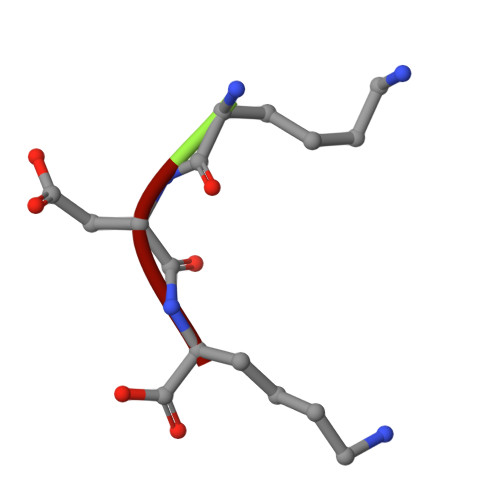> KDK>MDQTYSLESFLNHVQKRDPNQTEFAQAVREVMTTLWPFLEQNPKYRQMSLLERLVEPERVIQFRVVWVDDRNQIQVNRAWRVQFSSAIGPYKGGMRFHPSVNLSILKFLGFEQTFKNALTTLPMGGGKGGSDFDPKGKSEGEVMRFCQALMTELYRHLGADTDVPAGDIGVGGREVGFMAGMMKKLSNNTACVFTGKGLSFGGSLIRPEATGYGLVYFTEAMLKRHGMGFEGMRVSVSGSGNVAQYAIEKAMEFGARVITASDSSGTVVDESGFTKEKLARLIEIKASRDGRVADYAKEFGLVYLEGQQPWSLPVDIALPCATQNELDVDAAHQLIANGVKAVAEGANMPTTIEATELFQQAGVLFAPGKAANAGGVATSGLEMAQNAARLGW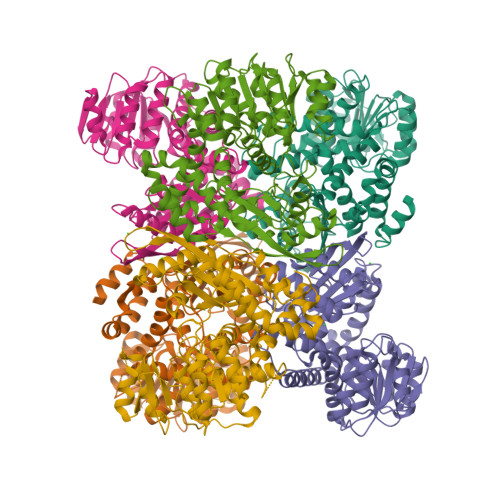KAEKVDARLHHIMLDIHHACVEHGGEGEQTNYVQGANIAGFVKVADAMLAQGVI[6x]>[6x]GHMTGAHERTFLAVKPDGVQRRLVGEIVRRFERKGFKLVALKLVQASEELLREHYAELRERPFYGRLVKY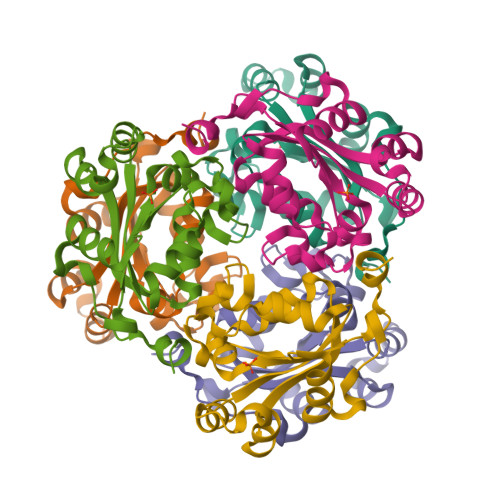MASGPVVAMVWQGLDVVRTSRALIGATNPADAPPGTIRGDFCIEVGKNLIHGSDSVESARREIALWFRADELLCWEDSAGHWLYE> SNIMKLDLQNKIAVVSGSTSGIGLGIAKGLASAGATVVVVGRKQAGVDEAIAHIRQSVPEASLRGVDADLTTEQGAAALFAAEPKADILVNNLGIFNDEDFFSVPDEEWMRFYQVNVLSGVRLARHYAPSMVEQGWGRIIFISSESGVAIPGDMINYGVTKSANLAVSHGLAKRLAGTGVTVNAVLPGP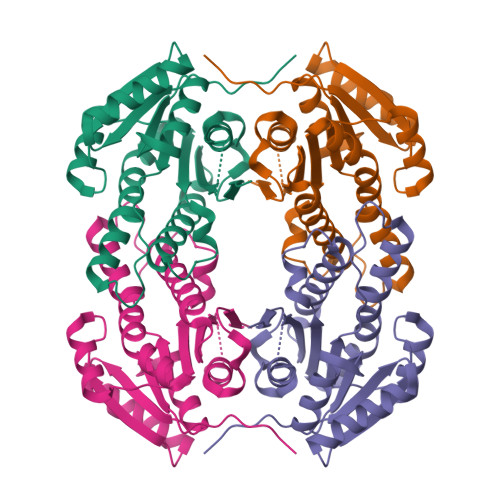TFTDGLENMLADAAAKAGRSTRDQADEFVKVLRPSSIIQRAAEVDEVANMVVYIASPLSSATSGAALRVDGGVVDTLV> DEVRKNLMDMFRDRQAFSEHTWKMLLSVCRSWAAWCKLNNRKWFPAEPEDVRDYLLYLQARGLAVKTIQQHLGQLNMLHRRSGLPRPSDSNAVSLVMRRIRKENVDAGERAKQALAFERTDFDQVRSLMENSDRCQDIRNLAFLGIAYNTLLRIAEIARIRVKDISRTDGGRMLIHIGRTKTLV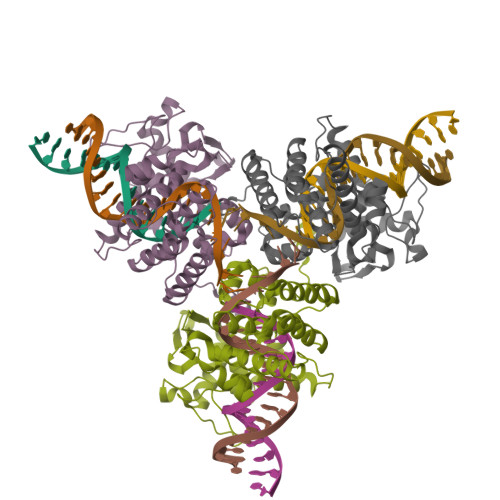STAGVEKALSLGVTKLVERWISVSGVADDPNNYLFCRVRKNGVAAPSATSQLSTRALEGIFEATHRLIYGAKDDSGQRYLAWSGHSARVGAARDMARAGVSIPEIMQAGGWTNVNIVMNFIRNLDSETGAMVRLLEDGD>GVEETTPQNMTCQEFMDMNPKSMTPVAFWVVNRNTDFSGGDYVDWHEV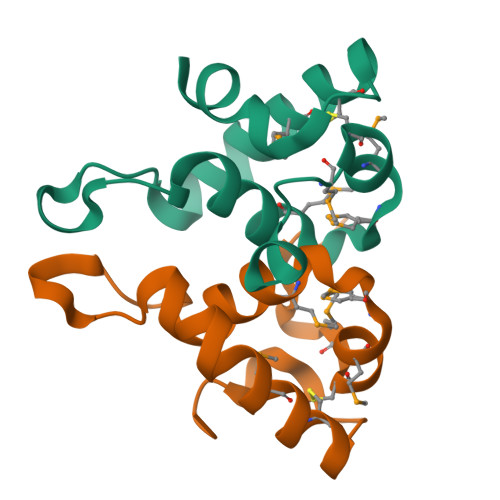ETVSVPKMLQECHKNPAAKLGDLSAVIKK[2x]>[4x]MGMESLLEKVLKEWKGHKVAVSVGGDHSFTGTLEDFDEEVILLKDVVD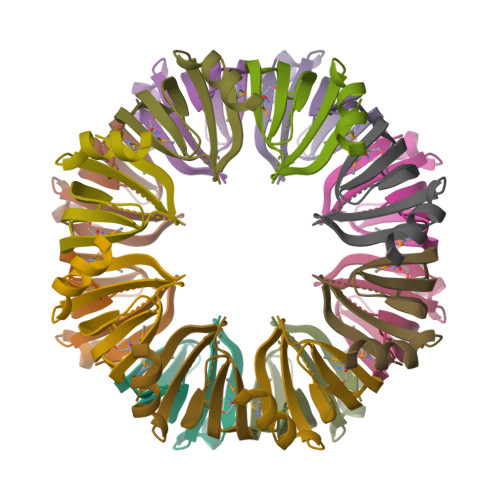VIGNRGKQMLIGLEDINWIMLLE>[2x]ADQTNPYKLMDEAAQKTFDRLKNEQPQIRANPDYLRTIVDQELLPYVQVKYAGALVLGQYYKSATPAQREAYFAAFREYLKQAYGQALAMYHGQTYQIAPEQPL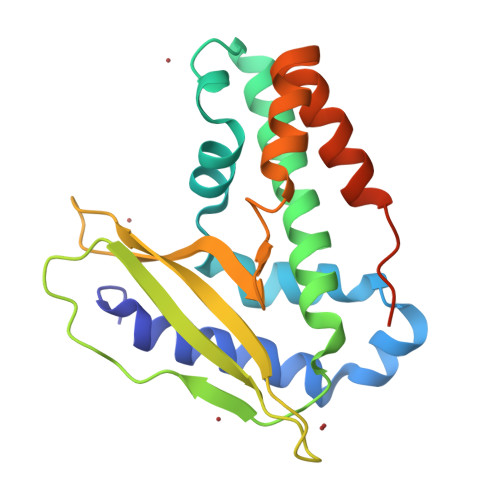GDKTIVPIRVTIIDPNGRPPVRLDFQWRKNSQTGNWQAYDMIAEGVSMITTKQNEWGTLLRTKGIDGLTAQLKSISQQKITLEEKKLEHHHHHH> MTDNPNKKTFWDKVHLDPTMLLILLALLVYSALVIWSASGQDIGMMERKIGQIAMGLVIMVVMAQIPPRVYEGWAPYLYIICIILLVAVDAFGAISKGAQRWLDLGIVRFQPSEIAKIAVPLMVARFINRDVCPPSLKNTGIALVLIFMPTLLVAAQPDLGTSILVALSGLFVLFLSGLSWRLIGVAVVLVAAFIPILWFFLMHDYQRQRVMMLLDPESDPLGAGYHIIQSKIAIGSGGLRGKGWLHGTQSQLEFLPERHTDFIFAVLAEELGLVGILILLALYILLIMRGLWIAARAQTTFGRVMAGGLMLILFVYVFVNIGMVSGILPVVGVPLPLVSYGGSALIVLMAGFGIVMS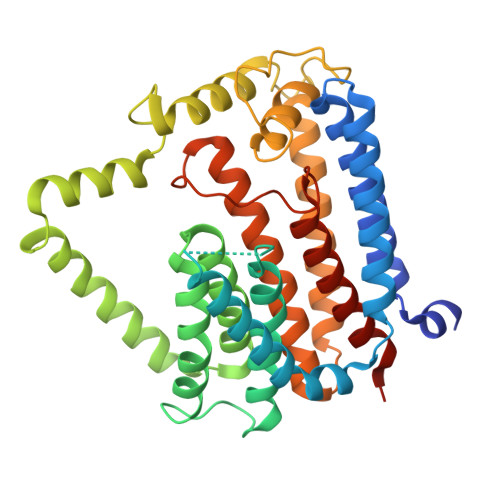IHTHRKMLSKSV>[2x]MGSSHHHHHHSSGLVPRGSVGGCLAKDGLQQSKCPDTTPKRRRASSLSRDAERRAYQWCREYLGGAWRRVQPEELRVYPVSGGLSNLLFRCSLPDHLPSVGEEPREVLLRLYGAILQGVDSLVLESVMFAILAERSLGPQLYGVFPEGRLEQYIP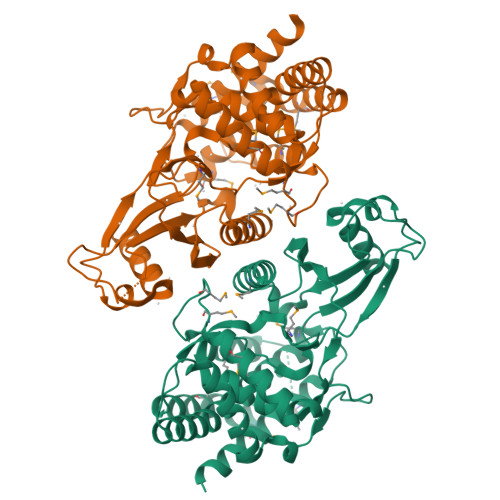SRPLKTQELREPVLSAAIATKMAQFHGMEMPFTKEPHWLFGTMERYLKQIQDLPPTGLPEMNLLEMYSLKDEMGNLRKLLESTPSPVVFCHNDIQEGNILLLSEPENADSLMLVDFEYSSYNYRGFDIGNHFCEWVYDYTHEEWPFYKARPTDYPTQEQQLHFIRHYLAEAKKGETLSQEEQRKLEEDLLVEVSRYALASHFFWGLWSILQASMSTIEFGYLDYAQSRFQFYFQQKGQLTSVHSSS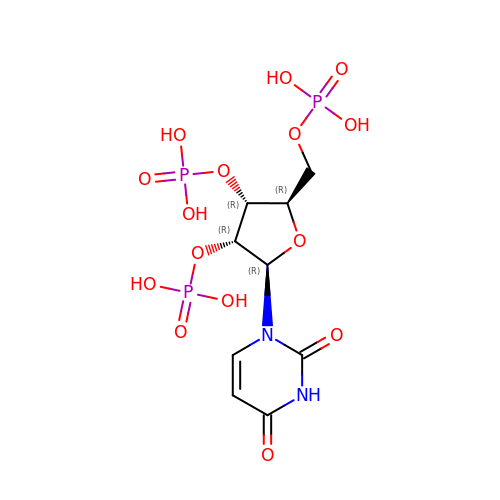[(2~{R},3~{R},4~{R},5~{R})-5-[2,4-bis(oxidanylidene)pyrimidin-1-yl]-3,4-diphosphonooxy-oxolan-2-yl]methyl dihydrogen phosphate | C9 H15 N2 O15 P3 | LGKMYXXYWOPMQI-XVFCMESISA-N>MEAGITGTWYNQLGSTFIVTA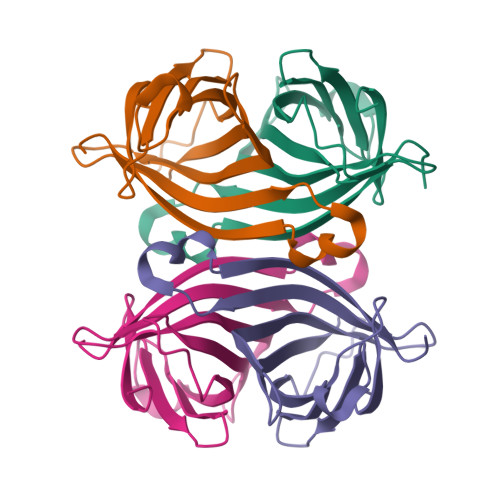GADGALTGTYIGARGNAESRYVLTGRYDSAPATDGSGTALGWTVAWKNNYRNAHSATTWSGQYVGGAEARINTQWLLTSGTTEANAWKSTLVGHDTFTKVKPSAAS[4x]> ALWQFNGMIKCKIPSSEPLLDFNNYGCYCGLGGSGTPVDDLDRCCQTHDNCYMQAMKLDSCKVLVDNPYTNNYSYSCSNNEITCSSENNACE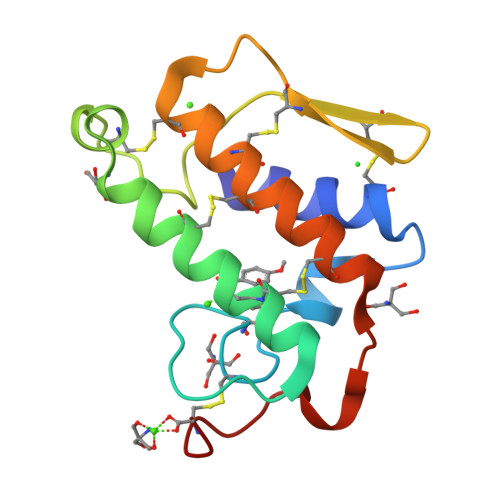AFICNCDRNAAICFSKVPYNKEHKNLDKMNC>[2x]MAHHHHHHMNLFQNAKFFTTVNHLKDLPDTPLEIAFVGRSNAGKSSAINTLTNHVRLAYVSK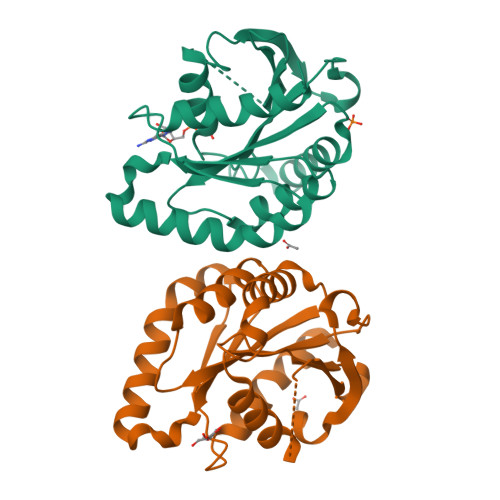TPGRTQHINFFELQNGNFMVDLPGYGYAQVPEAVRAHWVNLLGDYLRHRKQLIGLVLIMDARHPLKELDIRMLDFFHTTGRPVHILLSKADKLSKNEQIKTLSQVKKLLKPYSDRQNISVQLFSSLKKQGIDEANRTVGSWFDAADAAASSPEEN>GSHMEPPPKLVLDLERL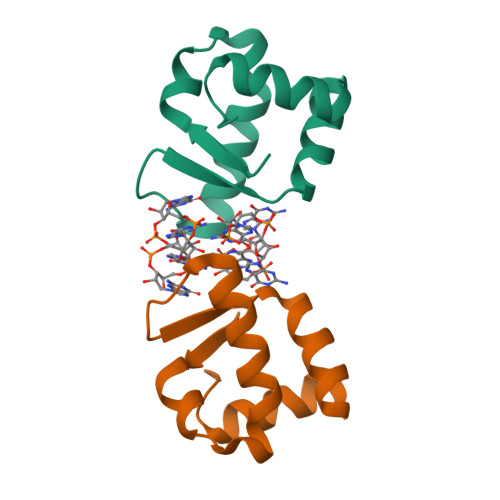AHVPQEKAGPLQRYAATIQSQRGDYNGKVLSIRQDDLRTLAVIYDQSPSVLTEQLISWGVLDADARRAVAHEEN[2x]N-({3-[({4-[(Z)-(2,4-DIOXO-1,3-THIAZOLIDIN-5-YLIDENE)METHYL]PHENYL}AMINO)METHYL]PHENYL}CARBONYL)-D-GLUTAMIC 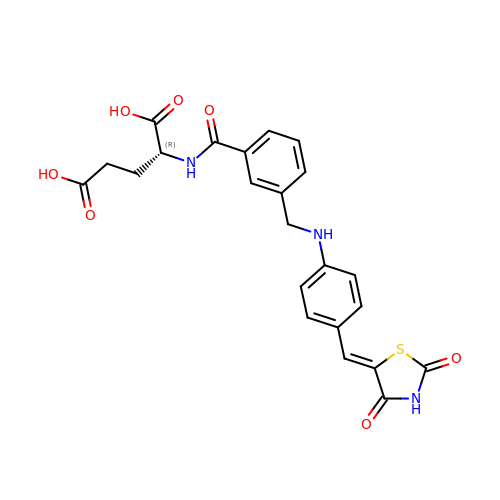ACID | C23 H21 N3 O7 S | YITBSJALJWUAQA-LVSMMTLPSA-N>[2x]GMNVDFINPFLDSLLNVLKTMANMELKPGKPNLKKDNLAKGDVSGLIGMVG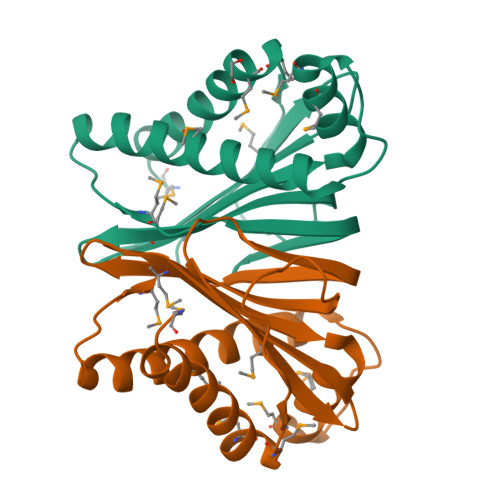PQTKGSLSITFEETLILEIMNKMLGEKPESIDEEVTDLVGELTNMVTGGAKNLLSDKGYEFDMATPIVVSGKNHTIAHKSDGQKIIMPFSSIYGTAYIEICFEG>VRTCLPCGPGGKGRCFGPSICCGDELGCFVGTAEALRCQEENYLPSPCQSGQKPCGSGGRCAAAGICCSP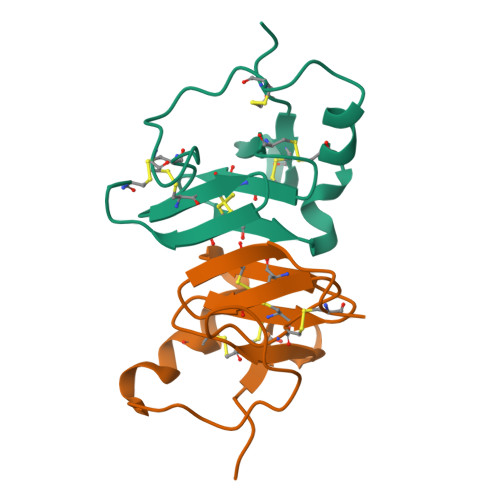DGCHEDPACD[5x]>[2x]DQGCAINFGKRELKCGDGIFIFRDSDDWLNKYSYYPEDPVKLASIVKASFEEGKCGLNSVDSLEHEMWRSRADEINAIFEENEVDISVVVQDPKNVYQRGTHPFSRIRDGLQYGWKTWGKNLVF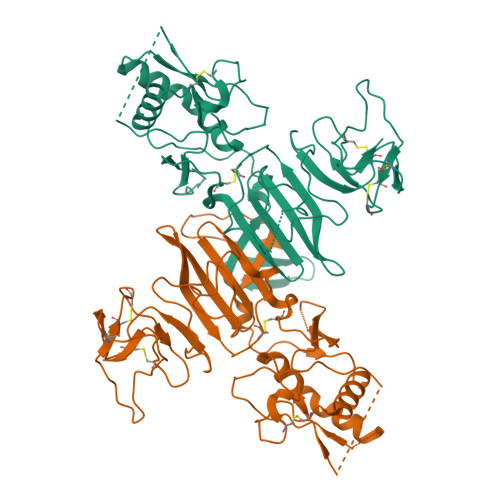SPGRKNGSFIIDGKSRKECPFSNRVWNSFQIEEFGTGVFTTRVYMDAVFEYTIDCDGSILGAAVNGKKSAHGSPTFWMGSHEVNGTWMIHTLEALDYKECEWPLTHTIGTSVEESEMFMPRSIGGPVSSHNHIPGYKVQTNGPWMQVPLEVKREACPGTSVIIDGNCDGRGKSTRSTTDSGKVIPEWCCRSCTMPPVSFHGSDGCWYPMEIRPRKTHESHLVRSWVTAHHHHHH>[2x]MEVDPRLYFENRSKFIQDQKDKGINPYPHKFERTISIPEFIEKYKDLGNGEHLEDTILNITGRIMRVSASGQKLRFFDLVGDGEKIQVLANYSFHNHEKGNFAECYDKIRRGDIVGIVGFPGKSKKGELSIFPKETILLSACLHMLPMKYGLKDTEIRYRQRYLDLLINESSRHTFVTRTKIINFLRNFLNERGFFEVETPMMNLIAGGANARPFITHHNDLDLDLYLRIATELPLKMLIVGGIDKVYEIGKVFRNEGIDNTHNPEFTSCEFYWAYADYNDLIKWSEDFFSQLVYHLFGTYKISYNKDGPENQPIEIDFTPPYPKVSIVEEIEKVTNTILEQPFDSNETIEKMINIIKEHKIELPNPPTAAKLLDQLASHFIENKYNDKPFFIVEHPQIMSPLAKYHRTKPGLTERLEMFICGKEVLN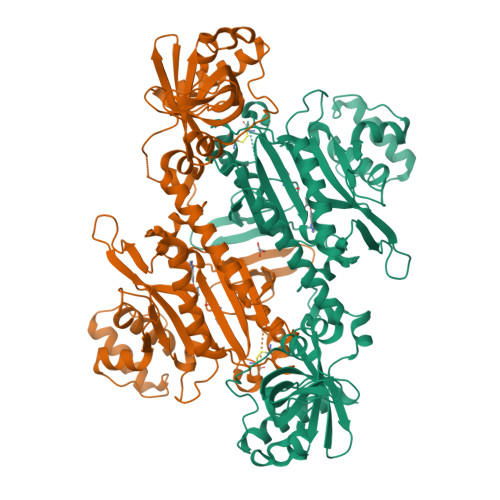AYTELNDPFKQKECFKLQQKDREKGDTEAAQLDSAFCTSLEYGLPPTGGLGLGIDRITMFLTNKNSIKDVILFPTMRPANGGHHHHHH(1R,2S,5S)-N-[(2S,3R)-4-amino-1-cyclobutyl-3-hydroxy-4-oxobutan-2-yl]-6,6-dimethyl-3-{3-methyl-N-[(1-methylcyclohexyl)carbamoyl]-L-valyl}-3-azabicyclo[3.1.0]hexane-2-carboxamide 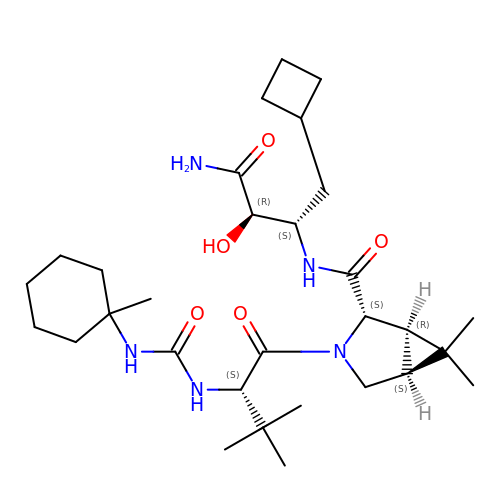| C30 H51 N5 O5 | WDNKLUIQDGESNW-CSCWZEDUSA-N>[2x]GSPSSVVRDVAIIGLSGRYPQAKNVDEFWNRLKEGKNCISEIPKDRWDWQSFFDEEKGKKESMYTKWGGFIDDMDKFDPLFFQISPKEAEEMDPQERLFLQEAYASIEDAGYTPTTLCESRKVGVFVGVMNGNYPTGATYWSIANRLSYLLNFQGPSVAVDTACSASLTAIHFALESLYSGTSECAIAGGVNLIVDPVHYMKLSALTMLSPSNQCKSFGDQADGFVDGEGVGAIVLKPLDKAIADGDHIYGVIKGSMMNAGGKTNGYTVPNPQAQAQLVADALQRANVHARTVSYLEAHGTGTELGDPIEVAGLTRAFEKDTQDKQFCALGSAKSNIGHCESAAGIAGVTKILLQLKHAQLVPSLHSRTLNPNIDFTKTPFVVQQELAEWRRPIVEINGTTNEYPRIAGISSFGAGGSNAHVIIEEYIPEEQKQSSLKITPQNPAIFVLSAKNAERLYEIVQQLLAFIQEHSLSDEHLADMAYTLQVGRVAMEERIAVIAGTMKELQQKLTAYVKGQEHIADLYRGQVNRNQEMLDILTSDDELEETIARWMERGKYSKLLDLWVKGLSIDWNKLYQEEQPGRISLPTYPFAKESYWTHARSVSSSTGVGVIHPFLHQNTSDFMEQRFSSMFTGQEFFLSDHVIKGQRVLPSAAYLEMARAAIQQATGGLDSERELEGLRFKNVVWTQPLAVGPEPVQAHIELYPEANGEIVFEIYSDSKQDRDQTTEIVHSQGSAVLCSIPDIPSFDLSVLQEQCSLRTLSAEQCYDAFKKMGVDYGPAHRGIEQILIGQEQVLAKLSLPSSVVKTQGQFGLHPSLLDAALQSSLGLMMATSDFSLILPF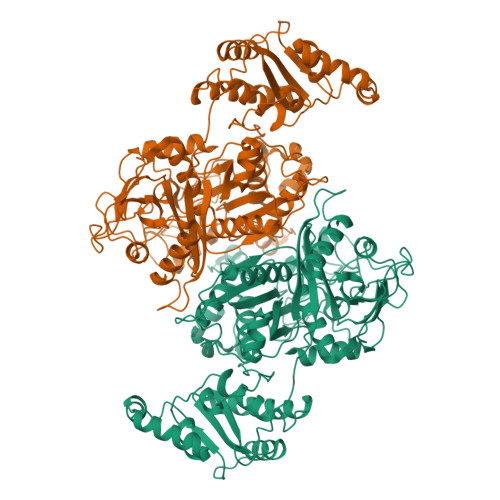ALEEMVIVGDCSSSMWALIRYREGSKAGDRVEKFDIDLCDENGNVQVRMKGFSTRKIANVSVRSEVEVPKASVPLEEEKAIDSSSLMEQATPYFKKLLSSVIKLPANKMEADASLEKYGVDSIVAMQMTKELEKQFGSLPKTLFFEYQTIKELTGYFLENYRENLMHILGMRENAEASLTQESEATMVDEVKAQTERRSKKRKSQRFASLRMETQPPKGALDIAIIGISGRYPQARNIHDFWKNLRDGKDCITEIPKDRWDHSLYFDEAKDKLGKSYSKWGGFIDGVDQFDPLFFHISPREAELMDPQERLFLQCVYETIEDAGYTRETLGKHEGLGGNVGVYVGVMYEEYQLYASAEQALGRALAIAGSPASIANRVSYFCNFHGPSMAVDTMCSSSLTGIHLACHSLQRGECEVAIAGGVNVSIHPNKYLYLSQGKFASSKGRCESFGEGGDGYVPGEGVGAVLLKPLARAIADGDHIYGVIKGSAINHGGKTNGYTVPNPHSQSRVIRRAFEEAGIHPRTVSYIEAHGTGTSLGDPIEIAGLTKTFQEYTKENQFCAIGSAKSNIGHGESAAGIAGLTKILLQMKYKRLVPSLHSRTLNPNIDFSKTPFVVQQELAEWKRPVIEIDGVTREYARIAGISSFGAGGANAHLVIEEYIEAEHRPPSSISSKNPAVIVLSAKNKDRLREQVQRLLSAIREQVLTDNDLAEIAYTLQVGREAMEERFAVIVKSISELEAKLTYYLKDEADSPDLFTGQVKRNKETMDVFAADEDLQQAIDTWITKGKYAKILQMWVQGLIFDWNKLYGDTKPRRISLPAYPFARERYWLPKVESQAIGLTAGEPAYLHPL>[2x]MFLVDSHCHLDGLDYESLHKDVDDVLAKAAARDVKFCLAVATTLPSYLHMRDLVGERDNVVFSCGV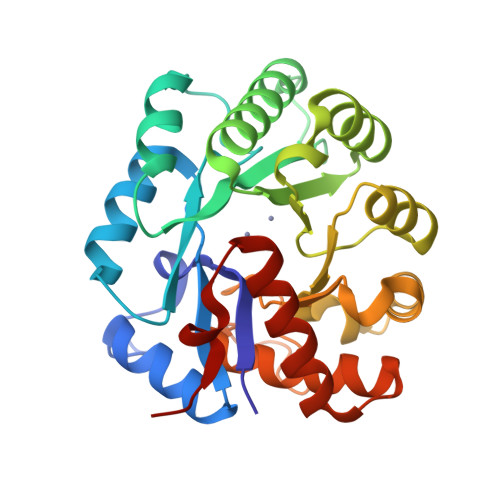HPLNQNDPYDVEDLRRLAAEEGVVALGETGLDYYYTPETKVRQQESFIHHIQIGRELNKPVIVHTRDARADTLAILREEKVTDCGGVLHCFTEDRETAGKLLDLGFYISFSGIVTFRNAEQLRDAARYVPLDRLLVETDSPYLAPVPHRGKENQPAMVRDVAEYMAVLKGVAVEELAQVTTDNFARLFHIDASRLQSIR>[2x]AGDLIGKVKGSHSVVVLGGGPAGLCSAFELQKAGYKVTVLEARTRPGGRVWTARGGSEETDLSGETQKCTFSEGHFYNVGATRIPQSHITLDYCRELGVEIQGFGNQNANTFVNYQSDTSLSGQSVTYRAAKADTFGYMSELLKKATDQGALDQVLSREDKDALSEFLSD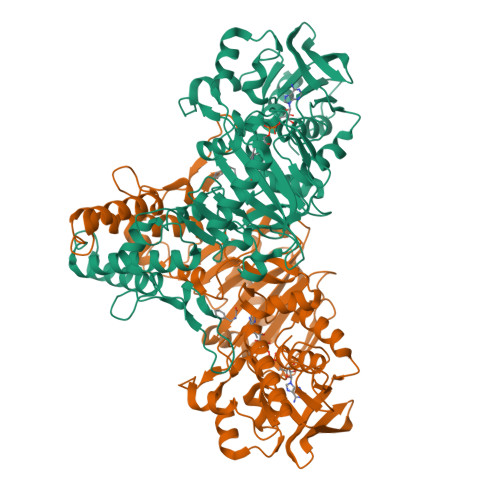FGDLSDDGRYLGSSRRGYDSEPGAGLNFGTEKKPFAMQEVIRSGIGRNFSFDFGYDQAMMMFTPVGGMDRIYYAFQDRIGTDNIVFGAEVTSMKNVSEGVTVEYTAGGSKKSITADYAICTIPPHLVGRLQNNLPGDVLTALKAAKPSSSGKLGIEYSRRWWETEDRIYGGASNTDKDISQIMFPYDHYNSDRGVVVAYYSSGKRQEAFESLTHRQRLAKAIAEGSEIHGEKYTRDISSSFSGSWRRTKYSESAWANWAGSGGSHGGAATPEYEKLLEPVDKIYFAGDHLSNAIAWQHGALTSARDVVTHIHERVAQEA> GAMAHGIPSQGKVTITVDEYSSNPTQAFTHYNINQSRFQPPHVHMVDPIPYDTPKPAGHTRFVCISDTRSRTDGIQMPYGDILLHTGDFTELGLPSEV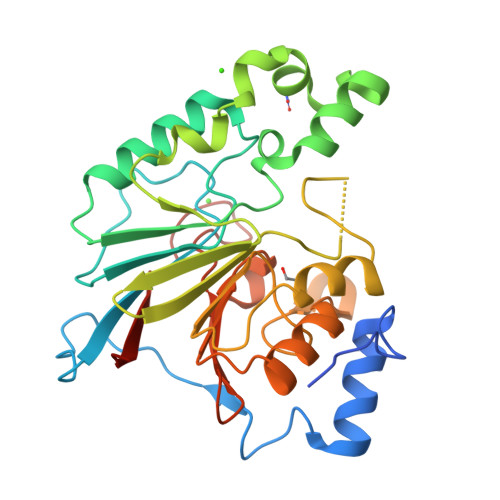KKFNDWLGNLPYEYKIVIAGNHELTFDKEFMADLVKQDYYRFPSVSKLKPEDFDNVQSLLTNSIYLQDSEVTVKGFRIYGAPWTPWFNGWGFNLPRGQSLLDKWNLIPEGTDILMTHGPPLGFRDWVPKELQRVGCVELLNTVQRRVRPKLHVFGGIHEGYGTMTDGYTTYINASTCTVSFQPTNPPIIFDLPNPQGS> TTHFTVTDQWGNVVSYTTTI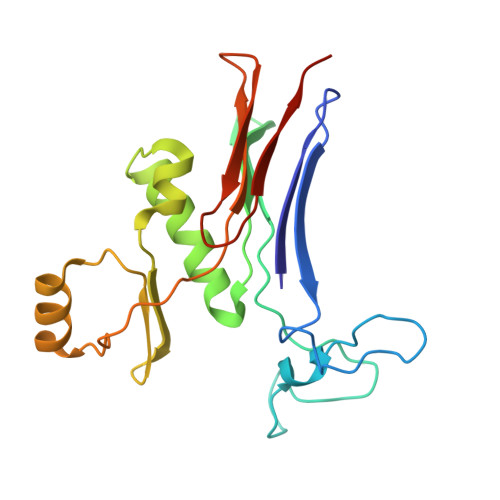EQLFGTGILVPGYGLFLNNELTDFDAIPGGANEVQPNKRPLSSMTPTIVFKDEKPVLTVGSPGGTTIIASVFQTILNYFEYGMSLQDAIEEPRIYTNSLTSYRYESGMPEDVRRKLNDFGHKFGSNPVDIGNVQSIFIDRENKTFMGVADSSRNGTAVGVNNKTSAE>[2x]MLILKGTKTVDLSKDELTEIIGQFDRVHIDLGTGDGRNIYKLAINDQNTFYIGIDPVKENLFDISKKIIKKPSKGGLSNVVFVIAAAESLPFELKNIA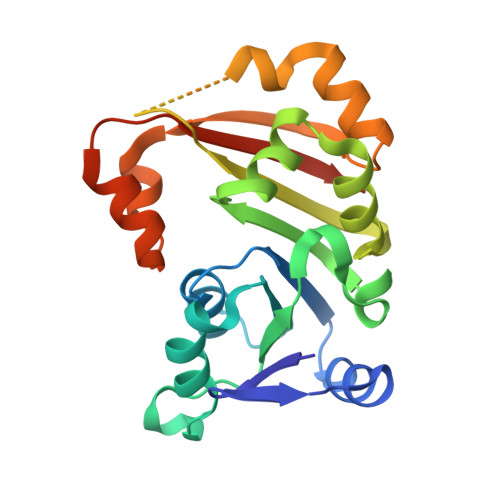DSISILFPWGTLLEYVIKPNRDILSNVADLAKKEAHFEFVTTYSDSYEEAEIKKRGLPLLSKAYFLSEQYKAELSNSGFRIDDVKELDNEYVKQFNSLWAKRLAFGRKRSFFRVSGHVSKHHHHHHH> GNPVTVVTATTGSKQNCTTGEGDYQLVQHEVLCSMKNTYEVLDFLGRGTFGQVVKCWKRGTNEIVAIKILKNHPSYARQGQIEVSILARLSTENADEYNFVRAYECFQHRNHTCLVFEMLEQNLYDFLKQNKFSPLPLKVIRPILQQVATALKKLKSLGLIHADLKPENIMLVDPVRQPYRVKVIDFGSASHVSK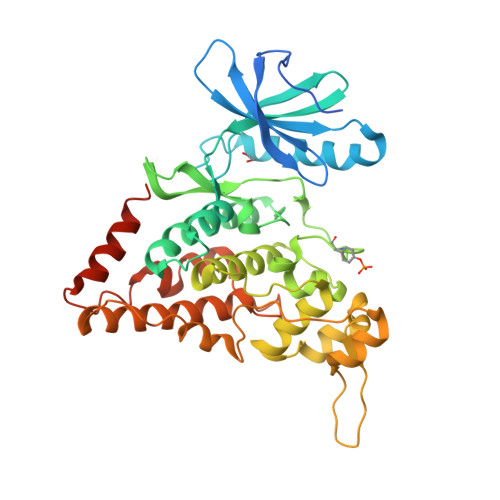TVCSTYLQSRYYRAPEIILGLPFCEAIDMWSLGCVIAELFLGWPLYPGALEYDQIRYISQTQGLPGEQLLNVGTKSTRFFCKETDMSHSGWRLKTLEEHEAETGMKSKEARKYIFNSLDDVAHVNTVMDLEGSDLLAEKADRREFVSLLKKMLLIDADLRITPAETLNHPFVNMKHLLDFPHSNHVKSCFHIMDICKSHLNSCDTNNHN> RPDFCELPAD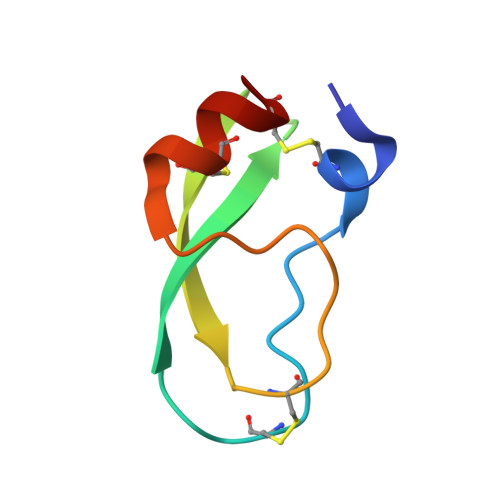TGPCRVRFPSFYYNPDEKKCLEFIYGGCEGNANNFITKEECESTCAA NITROGEN DIOXIDE | N O2 | 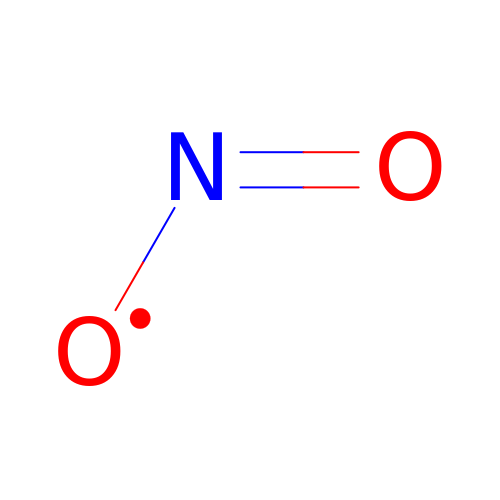IOVCWXUNBOPUCH-UHFFFAOYSA-N>[4x]MAVKEATSETKKRSGYEIITLTSWLLQQEQKGIIDAELTIVLSSISMACKQIASLVQRANISNLTGTQGAVNIQGEDQKKLDVISNEVFSNCLRSSGRTGIIASEEEDVPVAVEESYSGNYIVVFDPLDGSSNLDAAVSTGSIFGIYSPNDESLPDFGDDSDDNTLGTEEQRCIVNVCQPGSNLLAAGYCMYSSSVIFVLTIGKGVFVFTLDPLYGEFVLTQENLQIPKSGKIYSFNEGNYKLWDENL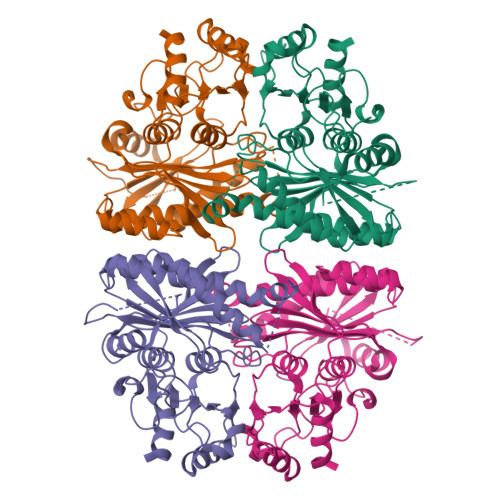KKYIDDLKEPGPSGKPYSARYIGSLVGDFHRTLLYGGIYGYPRDKKSKNGKLRLLYECAPMSFIVEQAGGKGSDGHQRVLDIQPTEIHQRVPLYIGSTEEVEKVEKYLA> GGAGUAGGCGUUGCGCAUUUUGUUGCUCAAAAGGCGACGAAACGCAAGGCAAUGCACGUCUGCGAUACACGAAAACAAUGCUAUUUGUUGAAAAUAUUGGAAUAAAGCAAAAGUCAUUGCCCGUCGCAAACGAAAGUGUGCUUCGGUAGCUAGGCUACCUGCUAGAGUCUCGCAAGGAUAAUAGCAAAGUCAAAGAGUAAAGCAGCUUAGACCUUUAGCGGGGUUUUCGUUAAUUGAAAAAUGGCUUAGUAGUUUGCGGCGUAACGAGUGGUUAGCGAUACUAACCGCGCAUGGUUGUUACUUGAAGGGAUUUGAG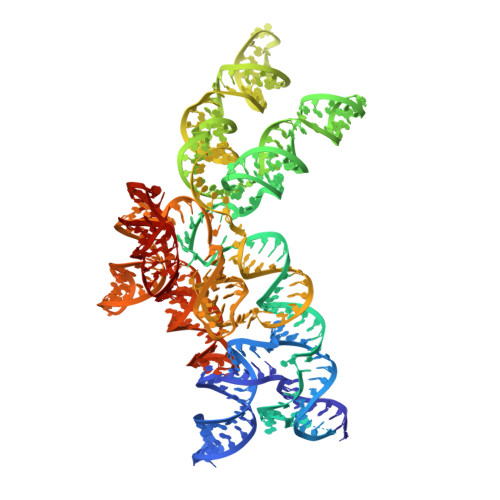UGGAUAAAAAACUAAAACAUAAGGUUUUGAAAGACAACUGACUAAACGUGUAAUCUCAGCGU>[2x]MDYN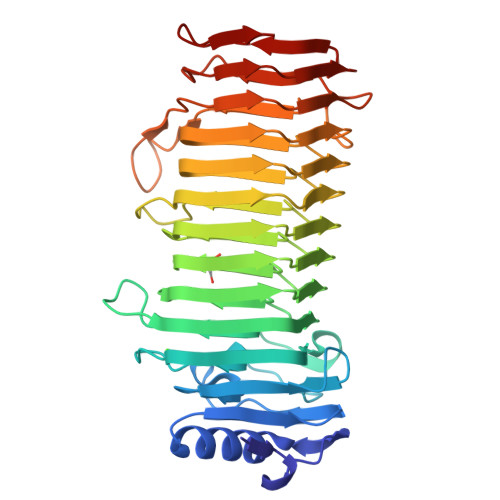VKDFGALGDGVSDDRASIQAAIDAAYAAGGGTVYLPAGEYRVSAAGEPGDGCLMLKDGVYLAGAGMGETVIKLIDGSDQKITGMVRSAYGEETSNFGMRDLTLDGNRDNTSGKVDGWFNGYIPGGDGADRDVTIERVEVREMSGYGFDPHEQTINLTIRDSVAHDNGLDGFVADYLVDSVFENNVAYANDRHGFNVVTSTHDFVMTNNVAYGNGSSGLVVQRGLEDLALPSNILIDGGAYYDNAREGVLLKMTSDITLQNADIHGNGSSGVRVYGAQDVQILDNQIHDNAQAAAVPEVLLQSFDDTAGASGTYYTTLNTRIEGNTISGSANSTYGIQERNDGTDYSSLIDNDIAGVQQPIQLYGPHSTVSGEP>VKIVTVKTKAYPDQKPGTSGLRKRVKVFQSSTNYAENFIQSIISTVEPAQRQEATLVVGGDGRFYMKEAIQLIVRIAAANGIGRLVIGQNGILSTPAVSCIIRKIKAIGGIILTASHNPGGPNGDFGIKFNISNGGPAPEAITDKIFQISKTIEEYAICPDLKVDLGVLGKQQFDLENKFKPFTVEIVDSVEAYATMLRNIFDFNALKELLSGPNRLKIRIDAMHGVVGPYVKKILCEELGAPANSAVNCVPLEDFGGHHPDPNLTYAADLVETMKSGEHDFGAAFDGDGDRNMILGKHGFFVNPSDSVAVIAANIFSIPYFQQTGVRGFARSMPTSGALDRVANATKIALYETPTGWKFFGNLMDASKLSLCGEESFGTGSDHIREKDGLWAVLAWLSILATRKQSVEDILKDHWHKFGRNFFTRYDYEEVEAEGATKMMKDLEALMFDRSFVGKQFSANDKVYTVEKADNFEYHDPVDGSVSKNQGLRLIFADGSRIIFRLSGTGSAGATIRLYIDSYEKDN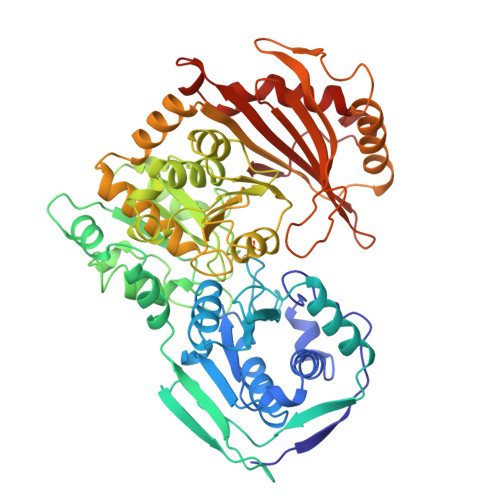AKINQDPQVMLAPLISIALKVSQLQERTGRTAPTVIT[2x]>[4x]HMCDSALTA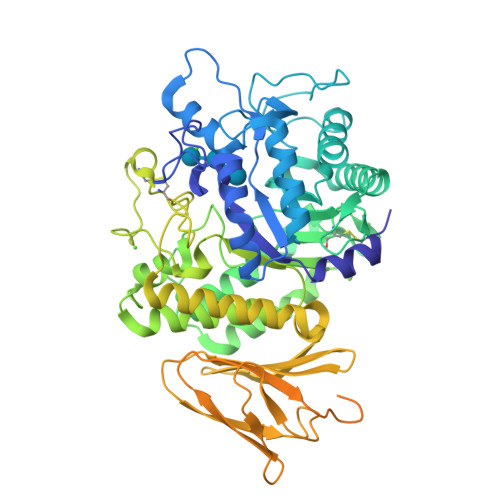QANDLRIYQVMVESFVNGDDAIGHGTGYGTSHHKGDLQGIIDSLDYIESLGMNAIWLTPIFDSIPVEGQDHWADRLDATGYFTSNYFAVDPRFGTMEQAKELVEKAHEKGLYVFFDGVFGHHKDNVVPSPEGRLPVGENNPVSYPESLAFYQEVATFWIEELKIDGWRLDQAYQVPTEAWTAIRASVDEASKSVTYVNSKGEAVNPLGYMVAQIWNNENYIKETGYGAEGEPALCSAFDFPVRYRVVETFAANENGIGNKGGKWLDEGMNLHRLYPSHAQPNLMLGNHDLVRFGDLLQRGNIASPEQAEYWERHKAALSFQAAYSGPITLYYGEEIGDELEGYAQKVEQDCAVQGLCDDHVARTSANIDGLTVNLNEKQRDLKQYVSQLMTLRAAHPALSRGERTNIVANETVYIDHKQADDDALIYMVSTTADQDTVELKASDIASDGQLVDLLTGKVHSAINGEYQISLAPFEAKFLLIETPSASGLTKVATVSAASSLIGEGFMAQCDNPTIEGDGPIGKTLYVVGDFADASWKQKPHRAYRYVGENTYQAVVDEKAGAFRMQYASKDWSPQFTADGLELTPGKTASLKRGGYGQDTAVTLPEAGQYVWSLKFTDSGDPEQIMVSKCP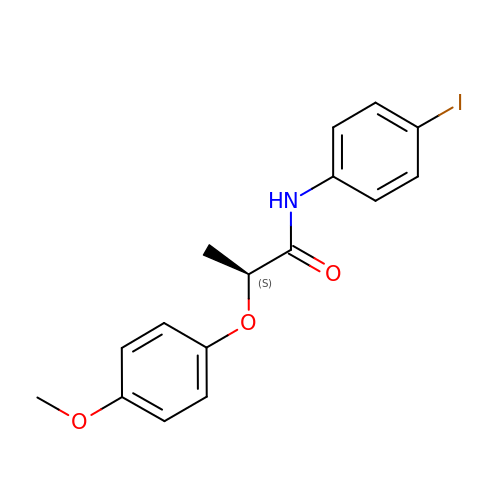(2~{S})-~{N}-(4-iodophenyl)-2-(4-methoxyphenoxy)propanamide | C16 H16 I N O3 | OTYVYTRAYJQPRW-NSHDSACASA-N> AWPKVQPEVNIGVVGHVDHGKTTLVQAITGIWTSKHSEELKRGMTIKLGYAETNIGVCESCKKPEAYVTEPSCKSCGSDDEPKFLRRISFIDAPGHEVLMATMLSGAALMDGAILVVAANEPFPQPQTREHFVALGIIGVKNLIIVQNKVDVVSKEEALSQYRQIKQFTKGTWAENVPIIPVSALHKINIDSLIEGIEEYIKTPYRDLSQKPVMLVIRSFDVNKPGTQFNELKGGVIGGSIIQGLFKVDQEIKVLPGLRVEKQGKVSYEPIFTKISSIRFGDEEFKEAKPGGLVAIGTYLDPSLTKADNLLGSIITLADAEVPVLWNIRIKYNLLERVVGAKEMLKVDPIRAKETLMLSVGSSTTLGIVTSVKKDEIEVELRRPVAVWSNNIRTVISRQIAGRWRMIGWGLVEI;> MIYSRSKLPSEGEILIATVKQVFDYGSYVSLDEYGGLQAFLPWSEVSSKWVKNIRDVLKENRKVIVKVIRVDRRKGTVDVSLKKVTDDERRKKNLQWKKIQRLDKILELVSQKLKLSEKDAWEQVAWKLEAKYGDPITAIEKAVKEGEKILIDAGVPEIWVKPLLEEASKHAEERKVKMSGLITVRTNEPLGVEKIKEVISKALE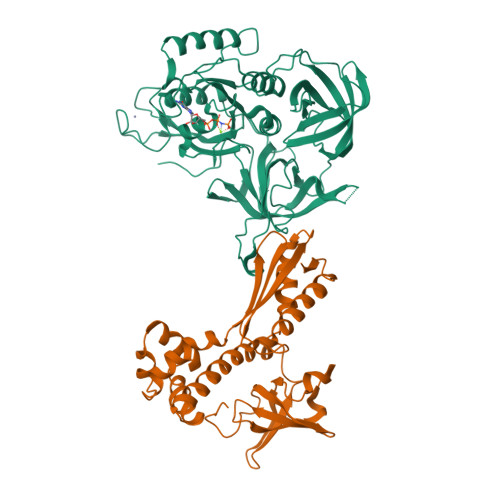NIEQDYESLLNIKIYTIGAPRYRVDVVGTNPKEASEALNQIISNLIKIGKEENVDISVVKK>XGELKAIAQEL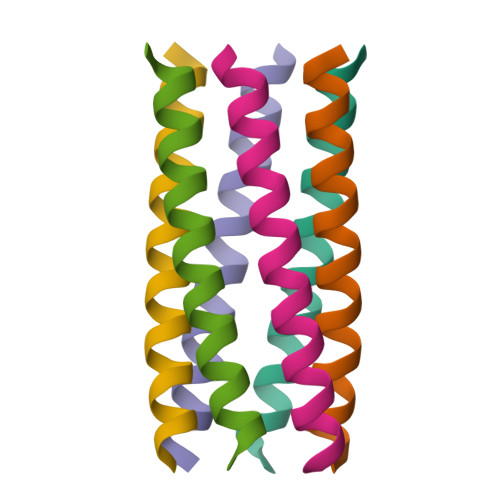KAIAKELKAIAWECKAIAQGAG[6x]3-[[(3~{S})-1-[2-(3,4-dimethoxyphenyl)ethyl]piperidin-3-yl]methyl]-7,8-dimethoxy-2,5-dihydro-1~{H}-3-benzazepin-4-one | C28 H38 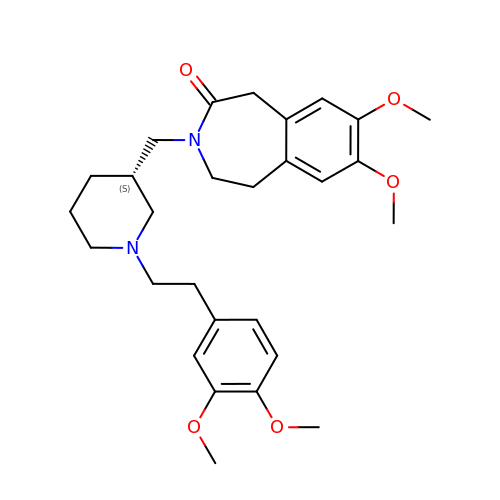N2 O5 | OBUFMJDDZTXJPY-NRFANRHFSA-N>GPLGSMPRKEKDFQGMLEYKKEDEQKLVKNLILELKPRGVAVNLIPGLPAYILFMCVRHADYLNDDQKVRSLLTSTINSIKKVLKKRGDDFETVSFWLSNTCRFLHCLKQYSGEEGFMKHNTSRQNEHCLTNFDLAEYRQVLSDLAIQIYQQLVRVLENILQPMIVSGMLEHETIQGVSGVKPTGLRKRTSSIADEGTYTLDSILRQLNSFHSVMCQHGMDPELIKQVVKQMFYIIGAITLNNLLLRKDMCSWSKGMQIRYNVSQLEEWLRDKNLMNSGAKETLEPLIQAAQLLQVKKKTDDDAEAICSMCNALTTAQIVKVLNLYTPVNEFEERVSVSFIRTIQMRLRDRKDSPQLLMDAKHIFPVTFPFNPSSLALETIQIPASLGLGFISRV[2x]

Type V myosin (MyoV) motors move protein complexes, organelles, vesicles, and mRNAs along actin cables. The C-terminal globular domain (GD) defines this class of myosins and mediates the majority of cargo interactions. In vertebrate Myo5a, the GD also mediates autoinhibition of ATPase activity in its cargo-free state. In this study, we describe the high-resolution X-ray structures of the GDs from human Myo5a and Myo5b as well as low-resolution SAXS-surface envelopes for all three human MyoV paralogs.

Indeed, a Myo5a fragment consisting of residues 1467–1855 (Myo5a (1467–1855)) was resistant to degradation and not prone to aggregation. By performing molecular replacement with the derivatized structure as template an atomic model was built with this native dataset at a resolution of 2.2 Å (Rwork = 0.22, Rfree = 0.26). The asymmetric unit contained two almost identical Myo5a molecules with a root mean square deviation for the c-α backbone atoms of 0.30 Å. Both molecules showed electron density for residues 1461 to 1855, with the exception of a predicted loop region ranging from residues 1640 to 1658 (loop I). The overall structural core of the Myo5a GD is hook-like shaped and its overall structural arrangement and connectivity is conserved in type V myosins. It consists of 11 tightly packed α-helices followed by an extended region that clamps the entire structure like a bracelet. The peptide chain ends with a short helix, and a C-terminal two-stranded anti-parallel beta-sheet that folds against the very N-terminal residues. Previously reported point mutations at residues I1512, M1515, and D1521 in the Myo5a GD are almost completely buried in the crystal structure. Thus, these Griscelli mutations are likely to destabilize the GD. Fitting our high-resolution X-ray structure of Myo5a GD into the low-resolution electron density of autoinhibited Myo5a allowed for only one possible orientation of the GD.>[2x]MVDIIIAEHAGFCFGVKRAVKLAEESLKESQGKVYTLGPIIHNPQEVNRLKNLGVFPSQGE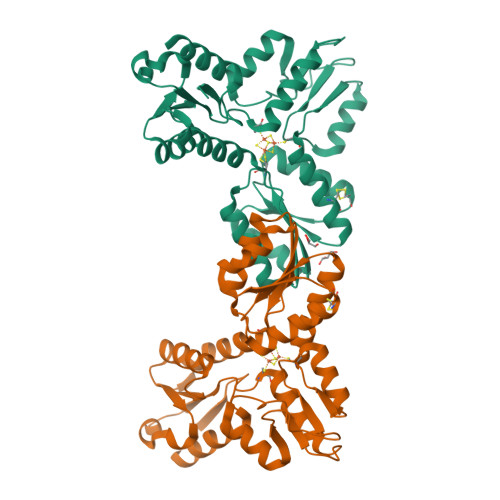EFKEGDTVIIRSHGIPPEKEEALRKKGLKVIDATCPYVKAVHEAVCQLTREGYFVVLVGEKNHPEVIGTLGYLRACNGKGIVVETLEDIGEALKHERVGIVAQTTQNEEFFKEVVGEIALWVKEVKVINTICNATSLRQESVKKLAPEVDVMIIIGGKNSGNTRRLYYISKELNPNTYHIETAEELQPEWFRGVKRVGISAGASTPDWIIEQVKSRIQEICEGQLVSSRSHHHHHH>SMNEKYVVTWDMLQIHARKLAQRLLPAEQWKGIIAVSRGGLVPAGILARELGIRYVDTVCISSYDHDNQRDLKVLKRA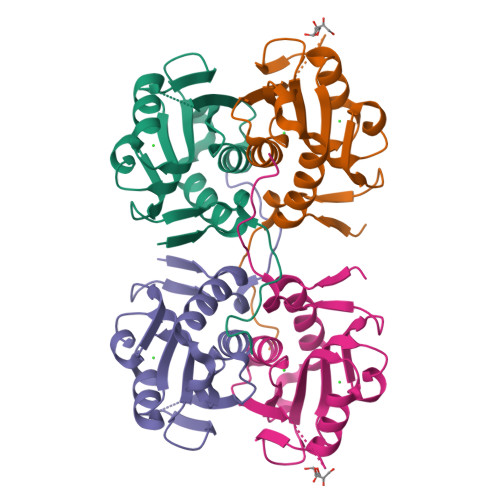EGDGEGFIVIDDLVDTGGTATAIREMYPKAHFVTIFAKPAGRPLVDDYVVDIPQNTWIFQPWDMAVTFVAPLSGK[2x]3-[(4-chlorobenzyl)amino]-6-(trifluoromethyl)quinoxaline-2-carboxylic acid | C17 H11 Cl F3 N3 O2 | 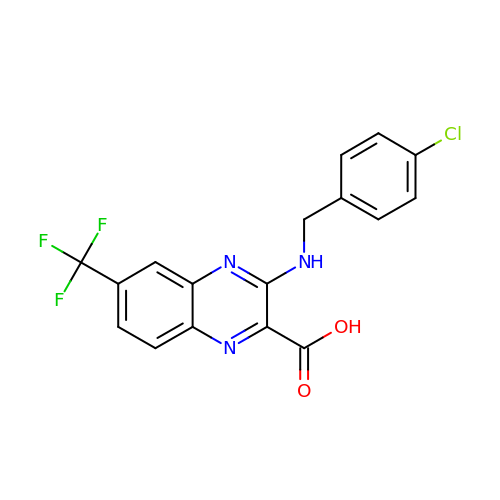JMDVDONAIBYSLS-UHFFFAOYSA-N>[2x]MPVDRILEAELAVEQKSDQGVEGPGGTGGSGSSPNDPVTNICQAADKQLFTLVEWAKRIPHFSSLPLDDQVILLRAGWNELLIASFSHRSIDVRDGILLATGLHVHRNSAHSAGVGAIFDRVLTELVSKMRDMRMDKTELGCLRAIILFNPDAKGLSNPSEVEVLREKVYASLETYCKQKYPEQQGRFAKLLLRLPALRSIGLKCLEHLFFFKLIGDTPIDTFLMEMLEAPHQLAGSGSGSHKILHRLLQDSSS;>GVQLTAAQELMIQQLVAAQLQCNKRSFSDQPKVTPWPLGADPASGSASQQRFAHFTELAIISVQEIVDFAKQVPGFLQLGREDQIALLKASTIEIMLLETARRYNHETECITFLKDFTYSKDDFHRAGLQVEFINPIFEFSRAMRRLGLDDAEYALLIAINIFSADRPNVQEPGRVEALQQPYVEALLSYTRIKRPQDQLRFPRMLMKLVSLR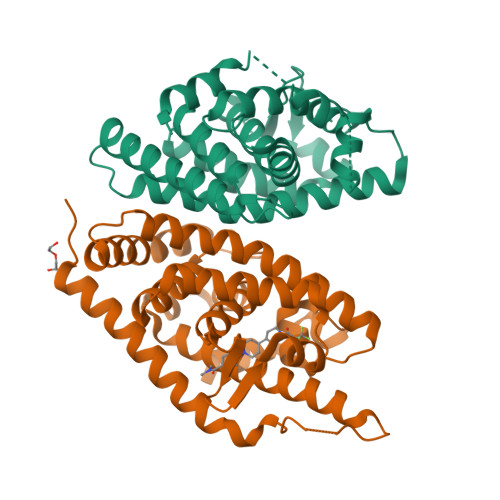TLSSVHSEQVFALRLQDKKLPPLLSEIWDVHEGSGSGSHKILHRLLQDSSS[2x]>[7x]SMGKQGQHAVSAYLADARRAL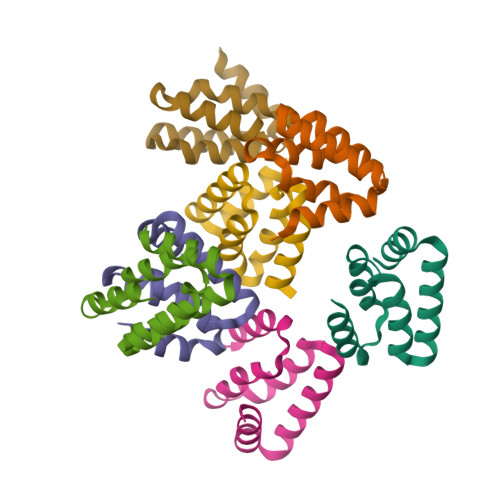GSAGCSQLLAALTAYKQDDDLDKVLAVLAALTTAKPEDFPLLHRFSMFVRPHHKQRFSQTCTDLTGRPYPGMEPPG> MSSQSSNTESLSRFPLWQVITPVRRKVILAMALAGLAALTSLGALLFLAWSLRDIRATPDAIPAWPLGGVIGCVVLTFVLRLQAFNTSHYAAFHLENILRSRLARKALQLPPGVLQQMGSGSVAKVMLDDVKSLHIFVADSTPLYARAIIMPLATIVILFWLDWRLAIATLGVLAFGSVVLVLARQRSENMAQRYHKAREQVSAAVIEFVQAMPVVRTFDSGSTSFLRYQRALEEWVDVLKTWYRKAGFSARFSFSILNPLPTLFVLIWSGYGLLHYG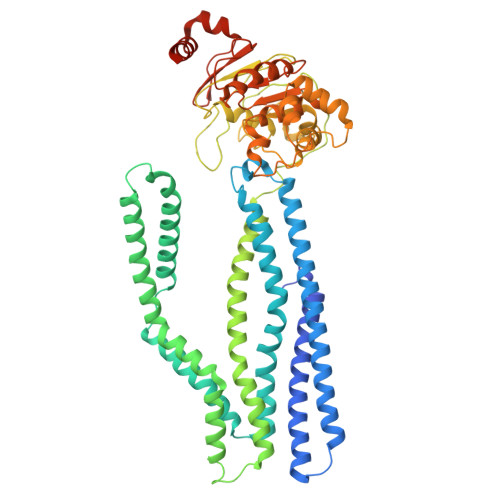SFDFIAWVAVLLLGSGMAEAVMPMMMLNNLVAQTRLSIQRIYQVLAMPELSLPQSDQQPQEASITFEQVSFHYPQARTGAALQEVSFHVPAGQIVALVGPSGAGKSTVARLLLRYADPDKGHIRIGGVDLRDMQTDTLMKQLSFVFQDNFLFADTIANNIRLGAPDTPLEAVIAAARVAQAHDFISALPEGYNTRVGERGVFLSGGQRQRITIARALLQDRPILVLDEATAFADPENEAALIKALAAAMRGRTVIMVAHRLSMVTQADVILLFSDGQLREMGNHTQLLAQGGLYQRLWQHYQQAQHWVPGGTQEEVVENERQ> GAMGSSTRDYEIQRERIELGRCIGEGQFGDVHQGIYMSPENPALAVAIKTCKNCTSDSVREKFLQEALTMRQFDHPHIVKLIGVITENPVWIIMELCTLGELRSFLQVRKYSLDLASLILYAYQLSTALAYLESKRFVHRDIAARNVLVSSNDCVKLGDFGLSRYMEDSTYYKA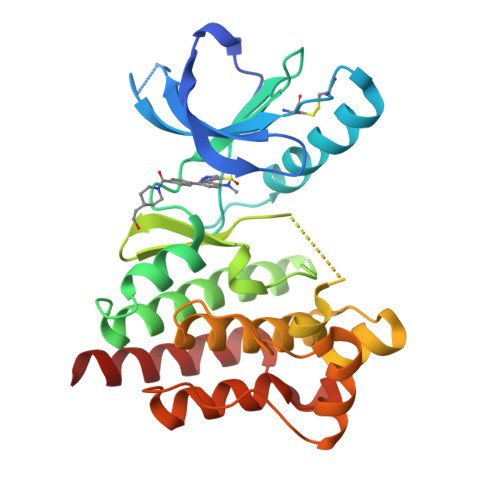SKGKLPIKWMAPESINFRRFTSASDVWMFGVCMWEILMHGVKPFQGVKNNDVIGRIENGERLPMPPNCPPTLYSLMTKCWAYDPSRRPRFTELKAQLSTILEEEKAQ> GSMDSSPNEFLNKVIGKKVLIRLSSGVDYKGILSCLDGYMN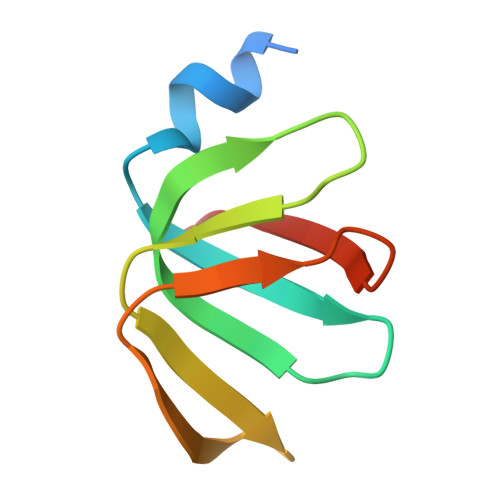LALERTEEYVNGKKTNVYGDAFIRGNNVLYVSALDD>[15x]ENSGGNAFVPAGNQQEAHWTINLKDADIREFIDQISEITGETFVVDPRVKGQVSVVSKAQLSLSEVYQLFLSVMSTHGFTVVAQGDQARIVPNAEAKTEAGGGQSAPDRLETRVIQVQQSPVSELIPLIRPLVPQYGHLAAVPSANALIISDRSANIARIEDVIRQLDQKGSHDYSVINLRYGWVMDAAEVLNNAMSRGQAKGAAGAQVIADARTNRLIILGPPQARAKLVQLAQSLDTPTARSANTRVIRLRHNDAKTLAETLGQISEGMKNNGGQGGEQTGGGRPSNILIRADESTNALVLLADPDTVNALEDIVRQLDVPRAQVLVEAAIVEISGDIQDAVGVQWAINKGGMGGTKTNFANTGLSIGTLLQSLESNKAPESIPDGAIVGIGSSSFGALVTALSANTKSNLLSTPSLLTLDNQKAEILVGQNVPFQTGSYTTNSEGSSNPFTTVERKDIGVSLKVTPHINDGAALRLEIEQEISALLPNAQQRNNTDLITSKRSIKSTILAENGQVIVIGGLIQDDVSQAESKVPLLGDIPLLGRLFRSTKDTHTKRNLMVFLRPTVVRDSAGLAALSGKKYSDIRVIDGTRGPEGRPSILPTNANQLFDGQAVDLRELMTE

In Gram-negative bacteria, the type 2 secretion system (T2SS) is composed of a pseudopilus assembly platform in the inner membrane and a secretin complex in the outer membrane. Pseudomonas aeruginosa has at least two T2SSs, with the ancestral nanomachine having a secretin complex composed of XcpQ. The T2SS containing XcpQ is responsible for the secretion of at least 19 substrates, most of them hydrolases ranging from proteases to hemolytic lipases that are critical for pathogenesis. In the T2SS secretins, each subunit consists of four N domains followed by the highly conserved secretin domain (Pfam PF00263), followed by an S domain.

After analysis of 18,000+ particles, class averages revealed that XcpQ is a pentadecameric secretin complex with no other symmetries observed in the two-dimensional (2D) class averages. At 3.6-Å resolution, the secretin complex was found to have 15-fold symmetry throughout the membrane-embedded region and through most of the domains in the periplasm. At 3.6-Å resolution, individual α-helices and β-strands were resolved throughout the upper part of the secretin structure and within the N3 domain, and the majority of the protein could be visualized. There is a relatively unstructured linker or hinge between the N3 and N2 domains (corresponding to residues 239 to 246 in the mature form of XcpQ), where the resolution of the structure starts to decline. Less well resolved density was present for the N1 domains, and no density for the N0 domains could be observed. The failure to identify these N domains raises the prospect that this region of the secretin complex, proximal to XcpP in the inner membrane, is not arranged in a uniform 15-fold symmetry. The disposition of the S domain in the XcpQ complex structure is equivalent to that of the other pilotin-dependent secretins. Structural comparisons with the Klebsiella-type secretin complex revealed a striking structural homology despite the differences in their sequence characteristics. We propose that a pseudo-6-fold symmetry exists in the proximal region of the N domains. The flexibility with which the features pack in order to transition from 15-fold to pseudo-6-fold symmetry provides insight into the mechanism for substrate entry into the T2SS, with the substrate-XcpP interactions competing for the XcpQ-XcpP interactions in order to gain entry into the XcpQ chamber; success in this competition would see the substrate be secreted via pseudopilus movements.> AMGVPCVEDEDFIQALDKMMLENLQQRSGESVKVH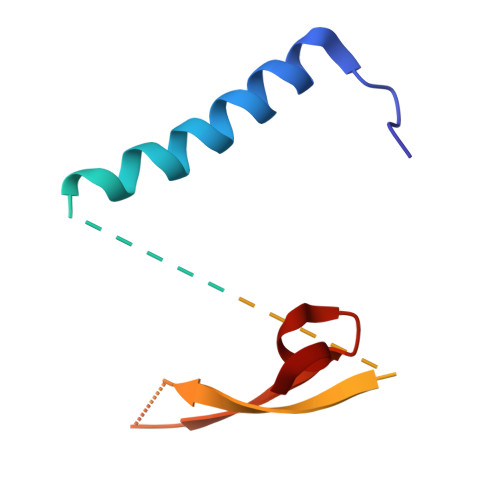QLDVAIPLHLKSQLRKGPPLGGGEGEAESADTMPFVMLTRKGNKQQFKILNVPMSSQLAANH> IVGGTNASLGEWPWQVSLQVKLVSQTHLCGGSIIGRQWVLTAAHCFDGIPYPDVWRIYGGILSLSEITKETPSSRIKELIIHQEYKVSEGNYDIALIKLQTPLNYTEFQKPISLPSKADTNTIYTNCWVTGWGYTKEQGETQNILQKATIPLVPNEECQKKYRDYV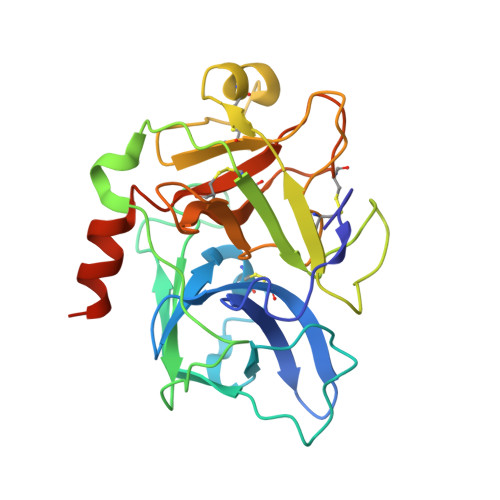INKQMICAGYKEGGTDACKGDSGGPLVCKHSGRWQLVGITSWGEGCARKDQPGVYTKVSEYMDWILEKTQSSDVRALETSSA Here, a high-throughput approach to determine room-temperature damage-free structures with excellent sample and time efficiency is demonstrated, allowing complexes to be characterized rapidly and without prohibitive sample requirements. We have applied this approach to crystals of two heme peroxidase enzymes: a multifunctional dehaloperoxidase from the marine annelid Amphitrite ornata (DHP-B; Barrios et al., 2014; Franzen et al., 2012; McCombs, Moreno-Chicano, et al., 2017; McCombs, Smirnova et al., 2017) and a dye-decolourizing peroxidase of industrial relevance from Streptomyces lividans (DtpAa). We also examine the challenging case of detecting nitrite binding to copper nitrite reductase from Achromobacter cycloclastes (AcNiR; Horrell et al., 2017), where the ligand displaces a water molecule bound in the active site. Our results cover several different ligand-binding scenarios, such as coordinate-bond formation to a heme iron (imidazole) or copper (nitrite) and noncoordinate ligand binding in a pocket (DHP ligands), with the latter being highly relevant to the binding of ligands to pharmacologically important proteins such as cytochromes P450.

Importantly, we used AcNiR–nitrite as a very challenging case to test the limitations of our approach as the nitrite ligand contains only three atoms and also displaces a water molecule upon binding. In addition, the water density in the native structure is disordered, with the presence of a second water molecule a possibility. Notably, refinement of AcNiR data and subsets versus the native AcNiR SFX structure produced clear positive difference map features for the nitrite atoms that are separated from the water molecule present in the native structure. Coot successfully located nitrite binding at the type 2 Cu active site in subsets of very few crystals, with 200 being the lowest number of crystals that were needed to successfully auto-find the nitrite ligand. Although Coot was unsuccessful at determining the ligand in the lowest crystal subset of only 100 crystals, positive electron density is still identifiable at the site where ligand binding is expected, although this did not allow for reasonable modelling of a ligand. For AcNiR, with cubic symmetry, the data remained essentially complete in all of the subset sizes analysed, with density for the nitrite ligand remaining apparent down to <200 indexed images. In AcNiR structures determined from single crystals, distinguishing between the electron-density features of active-site waters and nitrite is challenging and requires high-resolution data.

> DISTLPRVKVDLVKPPFVHAHDQVAKTGPRVVEFTMTIEEKKLVIDREGTEIHAMTFNGSVPGPLMVVHENDYVELRLINPDTNTLLHNIDFHAATGALGGGALTQVNPGEETTLRFKATKPGVFVYHCAPEGMVPWHVTSGMNGAIMVLPRDGLKDEKGQPLTYDKIYYVGEQDFYVPKDEAGNYKKYETPGEAYEDAVKAMRTLTPTHIVFNGAVGALTGDHALTAAVGERVLVVHSQANRDTRPHLIGGHGDYVWATGKFRNPPDLDQETWLIPGGTAGAAFYTFRQPGVYAYVNHNLIEAFELGAAGHFKVTGEWNDDLMTSVVKPASM> MSGDVFGPWYLGPIAHPAIGIRIPEIILTGILRAYKKRNVAGGLMLSFGRETAPEWVINAPPGKYEITRGHTGTSIRKYMTMAAEAAVKEGLVVEIEADHLTVAPSAAEAVKRISGVRTEYRMSEKELGESLNYIKAEIDEAVSTGYVNFYTIDTCFLIDYSAEEMSPGELESKFSTIFGDGAGDLLKRYVGRQFVYIGERGIPYCFTFTNEEVMRLALKYRESLKATKTICDYIKSKMSKPYGIEIAFDETPSLTKCKDMIFYLRELWEIGIKPDFIAPNIGFEKRKDYMGDLKVLEERVDKLAAIARAFGALLSIHSGSGSSPYSGKGIGTYEALLRATGGKIKYKISGVYIELLFELLASYPKGSKERGLYEQIFDDVYQFLKKEVEEEGVLASPELELQLKRYEEDVKNGVREERDPRADFFRYYSFVALNLRDSSGKRYLREAIVELYEEDRKFKERYDKEVEALTLRLIDGLKFENNI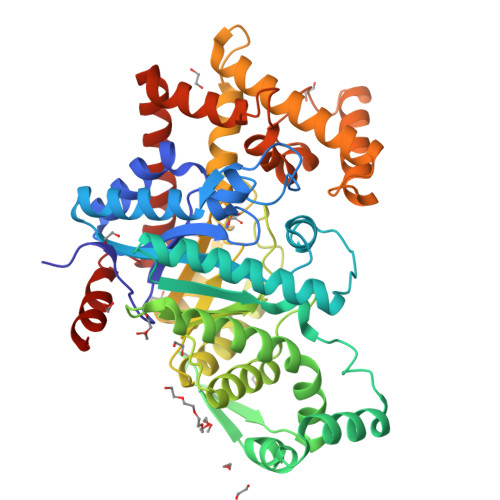INALAWIRQFHHHHHH>MKYQQLENLESGWKWAYLVKKHREGEAITRHIE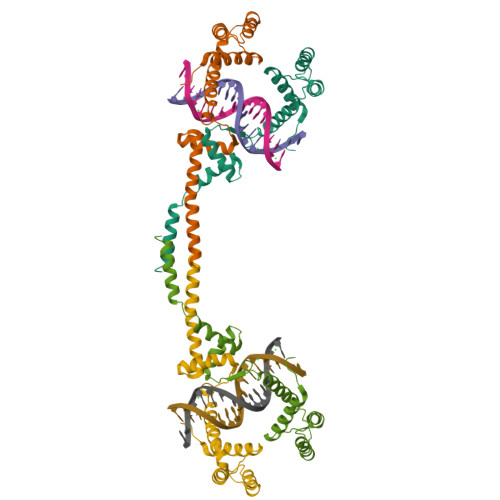NSAAQDAVEQLMKLENEPVKVQEWIDAHMNVNLATRMKQTIRARRKRHFNAEHQHTRKKSIDLEFLVWQRLAVLARRRGNTLSDTVVQLIEDAERKEKYASQMSSLKQDLKDILDKEV[2x]> MSSQKVFGITGPVSTVGATAAENKLNDSLIQELKKEGSFETEQETANRVQVLKILQELAQRFVYEVSKKKNMSDGMARDAGGKIFTYGSYRLGVHGPGSDIDTLVVVPKHVTREDFFTVFDSLLRERKELDEIAPVPDAFVPIIKIKFSGIS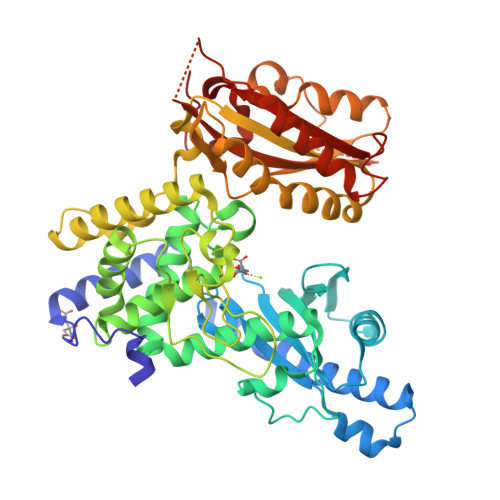IDLICARLDQPQVPLSLTLSDKNLLRNLDEKDLRALNGTRVTDEILELVPKPNVFRIALRAIKLWAQRRAVYANIFGFPGGVAWAMLVARICQLYPNACSAVILNRFFIILSEWNWPQPVILKPIEDGPLQVRVWNPKIYAQDRSHRMPVITPAYPSMCATHNITESTKKVILQEFVRGVQITNDIFSNKKSWANLFEKNDFFFRYKFYLEITAYTRGSDEQHLKWSGLVESKVRLLVMKLEVLAGIKIAHPFTKPFESSYCCPTEDDYEMIQDKYGSHKTETALNALKLVTDENKEEESIKDAPKAYLSTMYIGLDFNIENKKEKVDIHIPCTEFVNLCRSFNEDYGDHKVFNLALRFVKGYDLPDEVFDENEKRPS(3R)-3-hydroxy-L-aspartic acid | C4 H7 N O5 | 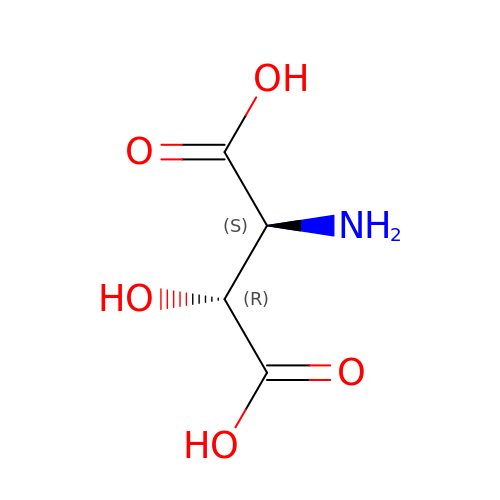YYLQUHNPNCGKJQ-NHYDCYSISA-N>LFGGLVLDVKRKAPWYWSDYRDALSLQCLASFLFLYCACMSPVITFGGLLGEATEGRISAIESLFGASMTGIAYSLFAGQPLTILGSTGPVLVFEKILFKFCKDYALSYLSLRACIGLWTAFLCIVLVATDASSLVCYITRFTEEAFASLICIIFIYEAIEKLIHLAETYPIHMHSQLDHLSLYYCRCALPENPNNHTLQYWKEHSIPTADVNWANLTVSECQEMHGEFIGSACGHHGPYTPDVLFWSCILFFATFIVSSTLKTFKTSRYFPTRVRSTVSDFAVFLTIFTMVILDFLIGVPSPKLQVPSVFKPTRDDRGWFISPIGPNPWWTVIAAIIPALLCTILIFMDQQITAVIINRKEHKLKKGCGYHLDLLVVAIMLGVCSLMGLPWFVAATVLSITHVNSLKLESECSAPGEQPKFLGIREQRVTGLMIFVLMGCSVFMTAVLKFIPMPV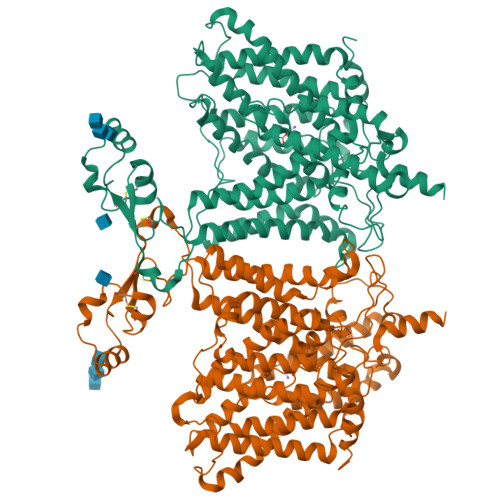LYGVFLYMGVSSLQGIQFFDRLKLFGMPAKHQPDFIYLRHVPLRKVHLFTLVQLTCLVLLWVIKASPAAIVFPMMVLALVFVRKVMDLCFSKRELSWLDDLMPESKKKKLDDAKK[2x]> ARRRRAEVRQLQPDLVYGDVLVTAFINKIMRDGKKNLAARIFYDACKIIQEKTGQEPLKVFKQAVE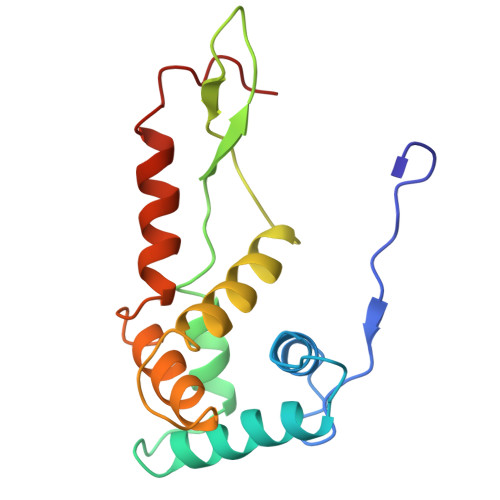NVKPRMEVRSRRVGGANYQVPMEVSRRQQSLALRWLVQAANQRPERRAAVRIAHELMDAAEGKGGAVKKKEDVERMAEANRAYAHYRW G-quadruplexes (G4s) are four-stranded secondary structures consisting of a core of multiple stacked ‘G-quartets’, also named guanine tetrads or simply tetrads, which are planar arrays of four guanines involving their Hoogsteen and Watson–Crick faces in eight hydrogen bonds overall. G4s are formed by single or multiple polynucleotide chains which have a rich content of contiguous guanines (G-runs or G-tracts), separated by loops which contain a variable number of nucleotides, usually other than guanines. Biologically relevant G-quadruplexes were first discovered in eukaryotic chromosomal telomeric DNA. Known G4-targeting ligands generally contain expanded π-systems and/or exhibit high levels of planarity to overlap with the G-quartet structures.

The derivatives bear a pyridine moiety connected by a hydrocarbon linker of varying length (n = 1–5, with n number of aliphatic carbon atoms) to the C13 position of the parent berberine. Only 2/Tel12 and 4/Tel12 adducts produced crystals suitable for diffraction analysis. The quadruplex adopts the expected bimolecular propeller conformation with four stacked quartets overall: three guanine quartets and a TATA quartet located at the 5′-end. The ligand 4 is lodged in the binding site at approximately a 3.4 Å π-stacking distance from both the GGGG and TATA tetrads. The berberine core gives π-stacking with the A2 adenine at the 5′-end, as well as with G5 and G11 at the 3′-end. The charged nitrogen atom points toward the groove, while the functionalized carbon points toward the central channel, so that the aliphatic pendant stretches and locates the pyridine ring just in contact with the second symmetry-related adenine on one side, and with the symmetry-related G5 on the other. 4 is involved in additional water-bridged H-bond contacts with the DNA polymer. The HOH-2 molecule bridges a C–H group at a long distance from pyridine (4.0 Å), and the phosphoester (2.9 Å) and ribose (3.0 Å) oxygens from T1, while the HOH-1 water molecule bridges a G5 phosphate oxygen (2.5 Å) and one oxygen from the benzodioxole group of the berberine core (2.3 Å). In addition to the H-bonds given by the benzodioxole group, the 4 structure confirms the structural features previously evidenced by the crystal structures of berberine and other C-13 berberine derivatives with Tel23 and Tel12. Several dark red spots are localized on the surface of 4 in proximity to G5 and to the HOH-1 water molecule, indicating strong and localized interactions.

> TAGGGTTAGGGT>LAPVPSTVCPLRRKLWQNYRNLTFDPVSANRHFYLSRQDQQVKHLRQSRGPGGPGSFELWQVQCAQSFQAGHHYWEVRASDHSVTLGVSYPQLPRSRLGPHTDNIGRGPSSWGLCVQEDSLQAWHNGEAQRLPGVSGRLLGMDLDLASGCLTFYSLEPQTQPLYTFHALFNQPLTPV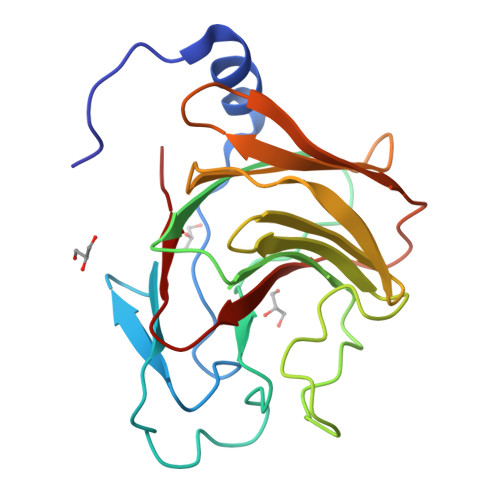FWLLEGRTLTLCHQ[3x]methyl (3S)-3-[(tert-butoxycarbonyl)amino]-4-oxopentanoate | C11 H19 N 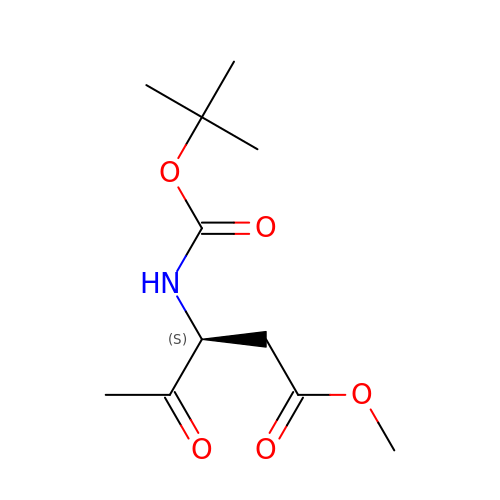O5 | QKEQESWFLCEUCV-QMMMGPOBSA-N>[2x]MSLSVTIVMIED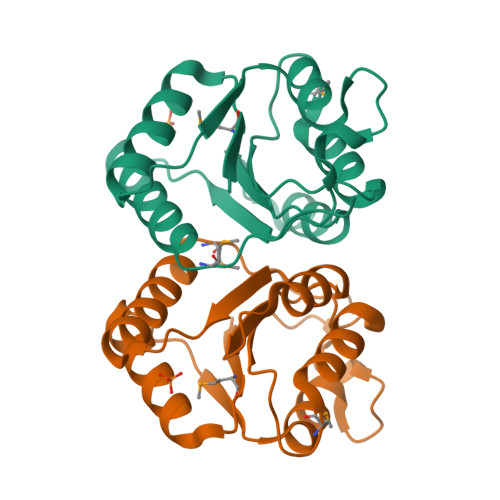DLGHARLIEKNIRRAGVNNEIIAFTDGTSALNYLFGDDKSGRVSAGRAQLVLLDLNLPDMTGIDILKLVKENPHTRRSPVVILTTTDDQREIQRCYDLGANVYITKPVNYENFANAIRQLGLFFSVMQVPETEGHHHHHH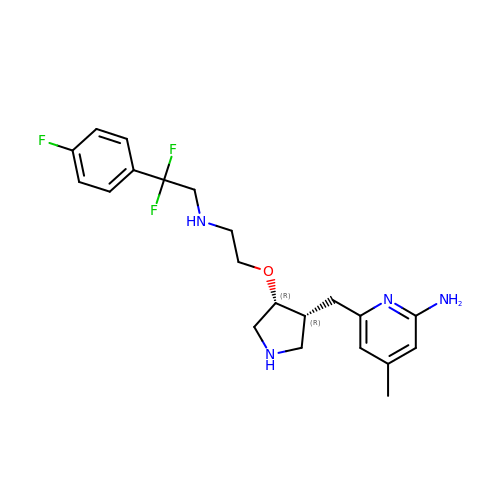6-{[(3R,4R)-4-(2-{[2,2-difluoro-2-(4-fluorophenyl)ethyl]amino}ethoxy)pyrrolidin-3-yl]methyl}-4-methylpyridin-2-amine | C21 H27 F3 N4 O | IFVHOVCZGYECQL-BEFAXECRSA-N>MKFFSLADEAEFKSIIISKNKAVDVIGSKLGGQVVSFSDEWFASAENLIQPTAPIRDPTRFVHSGAWYDGWETRRHNEMEYDWVIIKMGVAAAHIIGGEIDTAFFNGNHAPFVSIEALYDEGEEGNIVEDDSRWVEIVEKFECGPSQRHLFVRGNGLTKERFTHIKLKMYPDGGIARFRLYGRVVPPELKTKDHIIDLAYVCNGAVALKYSDQHFGSVDNLLLPGRGHDMSDGWETKRSRQPGHTDWAVIQLGRESSFIEKIIVDTAHFRGNFPQFITVEGCLK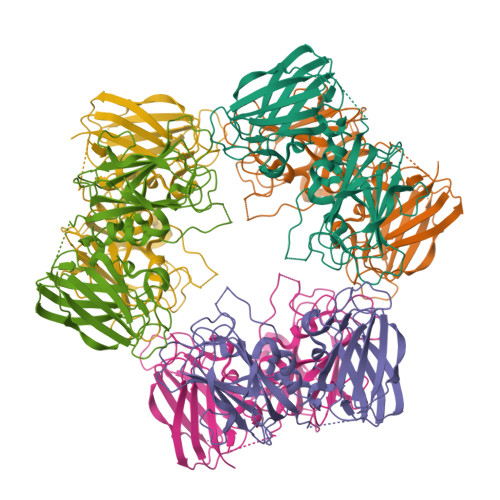ESESSENTGEGTWVELVGKSKTGPDKEHVYEIRKSIRVSHVKLTIIPDGGVKRIRVWGYHHHHHH[2x]>[2x]MQDRWREPAPPGEPLLEIHGGNRLSGAVRTSGFKHSLVTTVAAAATASAPVRIENCPDIVETAVLGEIFRAAGAHAHYDG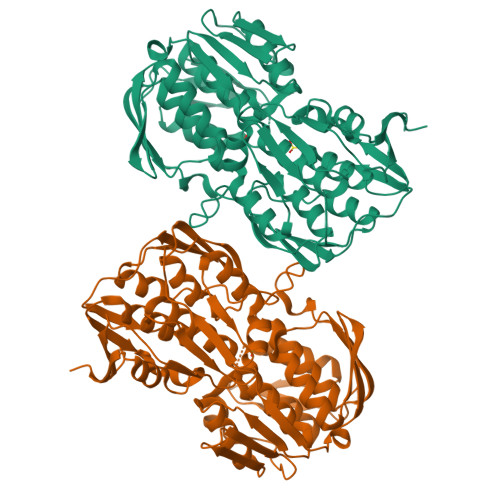ADETFTVDASAWDRAELPADLVGRIHGSLYLLPALVSRNGVARLSASGGCPIGEGPRGRPDEHLLDVMGRFGVTTRLTADGSVDLTAQRLTPCTIDMLDYTRNKALMSGPCYSGAVKTALLMGAVTHGTTTLQHPYLKPDVTDMVTVLRDLGADIEFAGPETWVIHGRGPESLHRPVDVTLIPDLIEVVTWICAGVLLADEPLRITGPGIDRAVHALAPEFDLLDRMGVRVDVGADEVTAHPLTKPLRPVEFTAMSRGVFSDSQPFLALLGAYAEGPTYIREAVWEHRFGFAPELEALGIRTAVDDTVLRVDGPCPPHRPGTDLRATDLRAAAVLLLAALAVPGRTTLRNHHHLARGYRDLVEDLVKLGADIRHTTAPDVRPKPPAGAGVDPAHHHHHH> KNTAN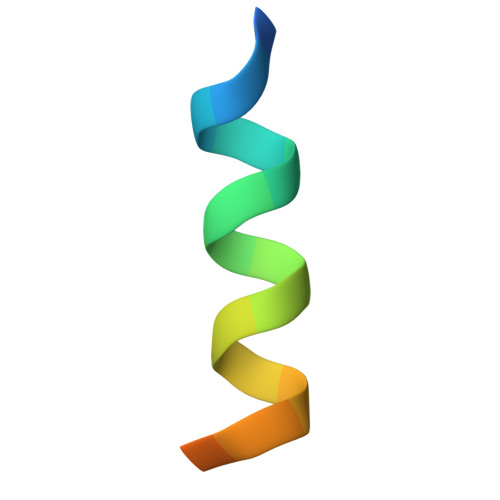IAKERLQIIVAERRR> SNAHMAPSAKDSEPATSCAAKKDSLNNYLWDLQYDKT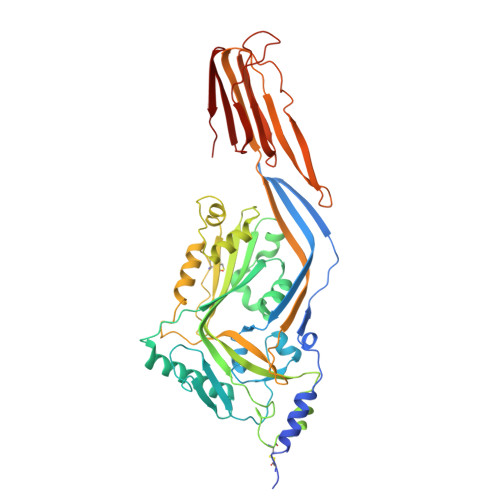NILARHGETIENKFSSDSFNKNGEFVVVEHQKKNITNTTSNLSVTSANDDRVYPGALFRADKNLMDNMPSLISANRAPITLSVDLPGFHGGESAVTVQRPTKSSVTSAVNGLVSKWNAQYGASHHVAARMQYDSASAQSMNQLKAKFGADFAKIGVPLKIDFDAVHKGEKQTQIVNFKQTYYTVSVDAPDSPADFFAPCTTPDSLKNRGVDNKRPPVYVSNVAYGRSMYVKFDTTSKSTDFQAAVEAAIKGVEIKPNTEFHRILQNTSVCAVILGGSANGAAKVCTGNIDTLKALIQEGANLSTSSPAVPIAYTTSFVKDNEVATLQSNSDYIETKVSSYRNGYLTLDHRGAYVARYYIYWDEYGTEIDGTPYVRSRAWEGNGKYRTAHFNTTIQFKGNVRNLRIKLVEKTGLVWEPWRTVYDRSDLPLVRQRTISNWGTTLWPRVAETVKND>[4x]MGSSHHHHHHSQDLENLYFQGGSTRLSLEAMLAERAMVARQDLAGLKRKLAGADRVLAPQSPEQCGRESAQAQARSVTSELKSAVKEAQGLEHQTLDFLEQLGEYPVCGILHGDHPVHPSGTHNNNGKVSVKRQFAAGVNTSDALTCAFRFEDSDLVRETALKTTYTDGTWAGFVQRLKMQTTRKCVQEKVSRKLLKQLFPYDPQKLVDVSGELSELVLGIKTNAIASAGPPYWRTKRDALPDMLDCVLPLLYDHIVRKDLTTLRNKHPELFLAECKNKTDRYEVESLGEKTRPYFSHPFHLSALVSVLSQSFSGALKIMTEDSTSFNAYGFSWTNGGAEDLAIWARQAGEAGKKPPRIACYGDDTDIYYRKDGKLYRICPDFKQMDGSVDATTIEAVVDYVVDAHVKQYPTARQFWEEVGKLWVEMATQSPFLIDGTKVYRKMQKDGLMTGVVGTTLFDTVKSALAYNDWADQLMFGSLNLLEEKYAIEF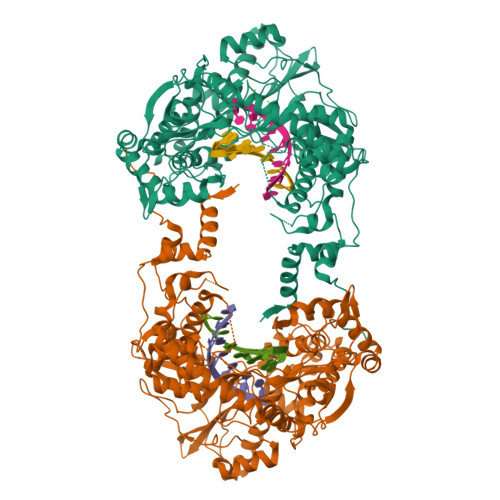FKNKHGLVIKEGTWKPALVNEDPGFGELWTEQKFLGLQLKVVRRENEKVYVPNLPFEDWLTMWVTPRSKYRSKETETMRERTLFDRARGLLVTGAVFDERARGLMGAVINSTAPEVVCMRVQEGGGRGAPPAYAFLTRDGVFEFPISDGYPSYDWVVSLYSRDHPCDMPRVFPEAATLIASYRKQVMDTRVVI>QQLSSNLWAAVRARGCQFLGPAMQEEALKLVLLALE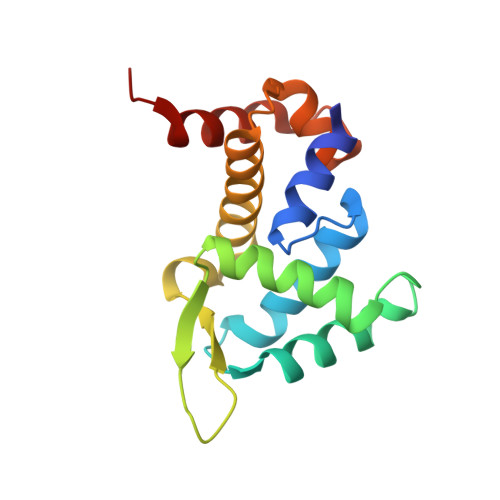DGSALSRKVLVLFVVQRLEPRFPQASKTSIGHVVQLLYRASCFKVTKRDEDSSLMQLKEEFRTYEALRREHDSQIVQIAMEAGLRIAPDQWSSLLYGDQSHKSHMQSIIDKLQTPA[2x]> GSTGSRPILEVPESVTGPWRGDVNLPCTYDPLQGYTQVLVRWLVQRGSDPVTIFLRDSSGDHIQQAQYQGRLHVSHRVPG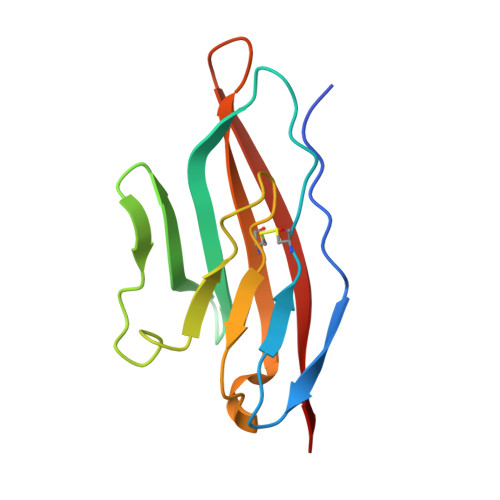DVSLQLSTLEMDDRSHYTCEVTWQTPDGNQVVRDRITELRVQK> GSPGISGGGGGILMDVNVGLSRLQSQAGAPVGTKGSNTRLAAKQRETLQAYDYLC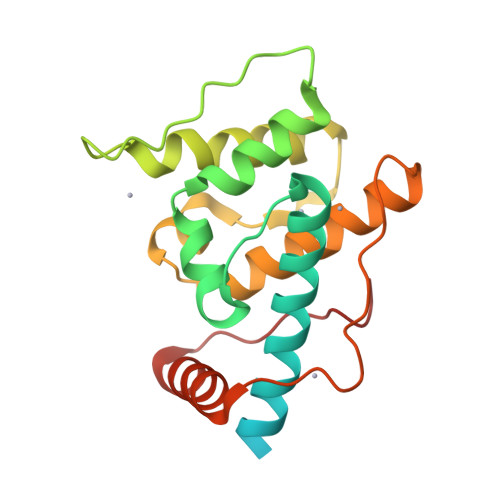RVDEAKKWIEECLGTDLGPTSTFEQSLRNGVVLALLVQKFQPDKLIKIFYSNELQFRHSDNINKFLDFIHGIGLPEIFHFELTDIYEGKNLPKVIYCIHALSYFLSMQDLAPPLIKSDENLSFTDEDVSIIVRRLRQSNVILPNFKAL> SVLSDFQEAVPTVVGIPDGTAVIGRSFRVSIPTDLIASSGEIIKVSAAGKEALPSWLHWDPHSHILEGLPLDTDKGVHYISVSAARLGANGSHVPQTSSVFSIEVYPEDHNEPQSVRAASSDPGEVVPSACAADEPVTVLTVILDADLTKMTPKQRIDLLNRMQSFSEVELHNMKLVPVVNNRLFDMSAFMAGPGNAKKVVENGALLSWKLGCSLNQNSVPDIRGVETPAREGAMSAQLGYPVVGWHIANKKPTLPKRLRRQI

Dystroglycan (DG), a ubiquitous membrane receptor belonging to the glycoprotein complex associated to dystrophin, plays a crucial role in the stability of the plasma membrane, especially in skeletal muscle tissues where it is highly expressed. A single gene, DAG1, encodes for a protein precursor, which is proteolytically cleaved in two subunits, alpha-dystroglycan (α-DG), located at the extracellular side of the plasma membrane where it binds several extracellular matrix proteins, and beta-dystroglycan (β-DG), which is a transmembrane protein that interacts with dystrophin in the cytoplasm. The molecular structure of the N-terminal region of α-DG (α-DG-Nt) was later determined at high resolution by X-ray crystallography, revealing the presence of two domains, an immunoglobulin-like (Ig-like) domain and a domain similar to the small subunit ribosomal protein S6 of T. termophilus (S6 domain), connected by a flexible loop. Noteworthy, it has been shown that α-DG-Nt is necessary for recruiting LARGE and some pathological conditions that are caused by missense mutations in the DAG1 map within the α-DG-Nt.

More recently, two additional mutations, namely V74I and D111N, located on the Ig-like domain surface facing the S6 domain within α-DG-Nt, have been found in a seven years old compound heterozygous patient, who displays mild muscular dystrophy and asymptomatic hyperCKemia. In particular, we focused on the murine α-DG-Nt region, fully validated as a model for the human counterpart, carrying the three pathological missense mutations V72I, D109N and T190M that correspond to their topological counterparts V74I, D111N and T192M in human DG. The crystal structures of D109N and V72I have been determined to a resolution of 1.70 Å and 1.80 Å, respectively. Similarly to what observed for T190M, residues 50–58 and 305–315, as well as residues 163–179 (V72I) or 164–179 (D109N), were missing in the D109N and V72I final models. That said, both D109N and V72I structures show the typical overall folding of α-DG-Nt. According to the refined crystallographic model, the pathological mutation Val72→Ile has no effect on the overall conformation of α-DG-Nt, but in this case also the local effects on the structure around the mutated residue are quite limited. On the contrary, the single mutant V72I shows a decrease both in Dmax (from 90 ± 3Å for WT to 80 ± 2Å for V72I) and in the Rg value (from 25.20 ± 0.04Å for the WT to 24.20 ± 0.04Å for V72I), pointing to a more compact shape as compared to the WT protein. In detail for V72I the profile is mainly unimodal characterized by a broader single peak: even if its maximum is slightly shifted to more compact models with Rg about 21–25 Å (60.4% of the total population), there is an increased fraction of extended models with intermediate Rg around 25–30 Å.Proteins attached to the surface of group A and group B streptococcal human pathogens that contain tandemly arrayed Rib domains have been associated with invasive infections and proposed as potential vaccine candidates. Here, we study Rib domains from Rib, R28, and from a surface protein from Lactobacillus acidophilus. Together, these 5 structures of homologous Rib domains, and further sequence analyses, show Rib is an example of domain atrophy, a rare event in domain structural evolution involving the loss of core secondary structure elements, and also reveal the remarkable structural malleability of this domain family. The structure, molecular dynamics simulations, and small angle X-ray scattering of a Rib domain pair suggest tandemly arrayed domains are likely to form an elongated rod on the bacterial cell surface, thus suggesting a possible mechanism of immune evasion mediated through domain number variation.

Structures of single Rib domains with ∼38% sequence identity were solved: RibR (S. agalactiae Rib; amino acids 230 to 308) and R28N (S. pyogenes R28; amino acids 230 to 307). The structure of RibR was determined by experimental phasing and refined at 1.7 Å resolution; the domain fold has a cuboidal structure consisting of a mixed 310/β fold comprising a 4-stranded β-sheet curved around 3 short 310-helices, with N and C termini pointing in opposite directions along the long axis of the anisometric fold. Analysis of the Guinier regions of both plots gives radius of gyration (Rg) values of 14.7 Å and 26.5 Å, and distance distribution [P(r)] functions determine maximum particle dimensions (Dmax) of 57 Å and 97 Å for RibR and Rib2R, respectively. These calculated Dmax values are consistent with our structural models (56 Å, RibR; 98 Å, Rib2R). RibR displays a Porod exponent of 1.8, consistent with a rod-like particle tending toward a “flat disk”-like shape. In the atrophy of the Ig-like RibL, a significant loss of the structure (∼20% compared to RibR/RibS) is involved, but the domains remain thermostable with melting temperatures (Tms) of 78 °C and 88 °C for RibL and RibS, respectively, and 71 °C for RibR. The Rib (RibR) structure revealed that the original Pfam analysis successfully predicted the C-terminal residues of the domain, but the N terminus of the HMM needed to be extended by ∼11 amino acids. This has been adjusted within the Pfam database, which now also includes new families representing the RibL and aRib domain.

>GPLGSDADKNDPAGKDQQVNVGETPKAEDSIGNLPDLPKGTTVAFETPVDTATPGDKPAKVVVTYPDGSKDTVDVTVKVVDPRT[2x]> TTLLNPYFGEFGGMYVPQILMPALNQLEEAFVSAQKDPEFQAQFADLLKNYAGRPTALTKCQNITAGTRTTLYLKREDLLHGGAHKTNQVLGQALLAKRMGKSEIIAETGAGQHGVASALASALLGLKCRIYMGAKDVERQSPNVFRMRLMGAEVIPVHSGSATLKDACNEALRDWSGSYETAHY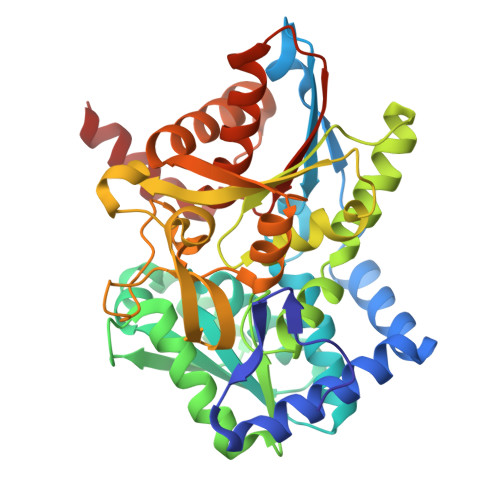MLGTAAGPHPYPTIVREFQRMIGEETKAQILDKEGRLPDAVIACVGGGSNAIGMFADFINDTSVGLIGVEPGGHGIETGEHGAPLKHGRVGIYFGMKAPMMQTADGQIEESYSISAGLDFPSVGPQHAYLNSIGRADYVSITDDEALEAFKTLCRHEGIIPALESSHALAHALKMMREQPEKEQLLVVNLSGRGDKDIFTVHDILKARG> MHHHHHHMRGTLRVGTEATFPPFGFKDENGKLVGFDIDLAKAIAKKLGVKVEFKPMDFDGIIPALQSGKIDVVIAGMTITEERKKQVDFSDPYFEAGQA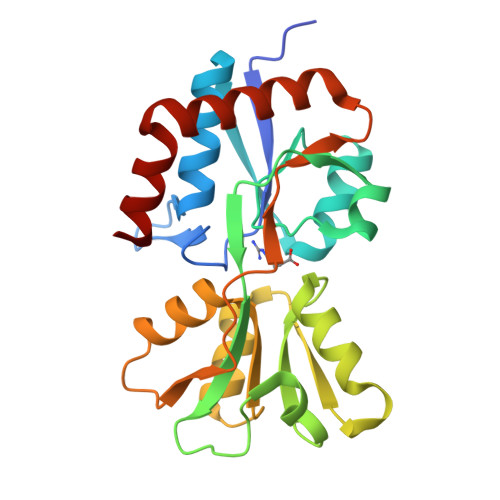IVVKKGNDSIKSLEDLKGKKVGVQLGSTSEQHVKKVAKDAGVKVKKFDNFSEAFQELKSGRVDAVVTDNAVALAYVKQNPNAGVKIVGETFSGEPYGIAVRKGNSELLEKINKALEEMKKDGTYDKIYEKWFGE Erythrosin | C20 H8 I4 O5 | 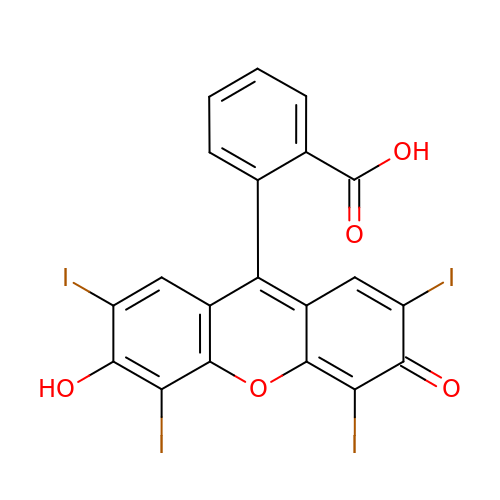LAINPTZBIXYTIZ-UHFFFAOYSA-N>[2x]MVAPLLKTLPFLAAAYAAELDLPNFSALNRRQDNSTSSSAGCSLDQ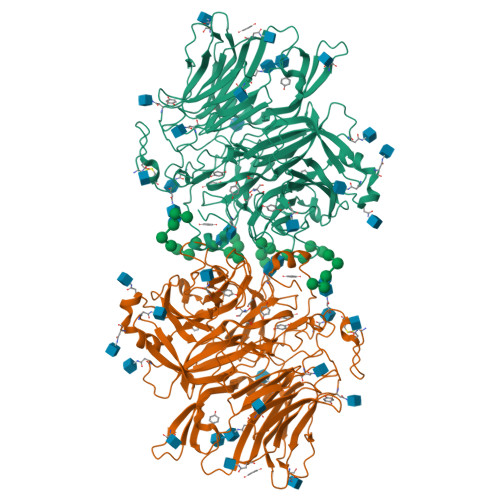TVAPGNLTLCGNATLFTTFRPKARFIAPEGWMNDPMGLYQRADGSIHAGYQSHPKHIQWGNISQGAAYSSDFTSWTDFNGSEGYKTIWPSQIYDIRGVFDGSIIKEGIDGYPTILYTSTSFGPLGATLNEAEGTETQSLAYTTDDGASWIKLGYGAGQNPVIYEWPETNLTGFRDPYVFQSPRLEALLANTTSITNATGDHFATISGGVHGDGARLFLYRQHTTGEFIKWTYLGPLVTTGYKESYGEWSGNYGINFETAGVTRLNPAGAAWDNGSDTTAVDFVTFGTEQGRADHQNHWPLWAAVDYEVRDNGSIEAVIAYSGVQDWGRSYAYASFPVEGYRQVSVGWIYEDDDNVILAKQFGYQGAFTLFRDLFVKVVENVSPSTPGLFEQASWSTKNSTDGMSVTVTTLGQRVVPETLAAYKGNSTVSTLAPVMLNESAAAYTPFSSQPTDRFYALTGSFEFGLNTTAKAGFRVLASEEEYTDIWFDPASENLTVVRTASSLIKSFGNDTELAKVKLYEIVGAESKTLNLTVFVDGSVIEIYANDEVALSTRAYPWLANSTGAGLLADGTTAGDVVGVSGLELWDGLVDAWPARPANTSQGLVWDGPTAAMYGLFAGY1-[4-(PYRIDIN-4-YLOXY)PHENYL]-3-[3-(TRIFLUOROMETHYL)PHENYL]UREA | 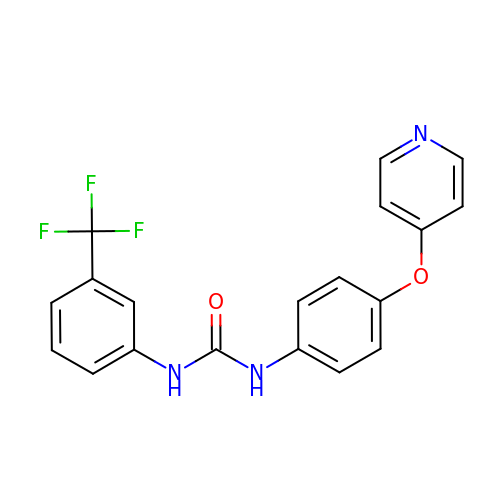C19 H14 F3 N3 O2 | DDDLGNOZDKDSEG-UHFFFAOYSA-N> MRSDGRKEDQLRPVSIQRDFLEYPEGSCLISFGKTKVICTASVIENVPNWLKGKGQGWITAEYSMLPRATQQRTIRESVQGRIGGRTHEIQRMIGRAMRTA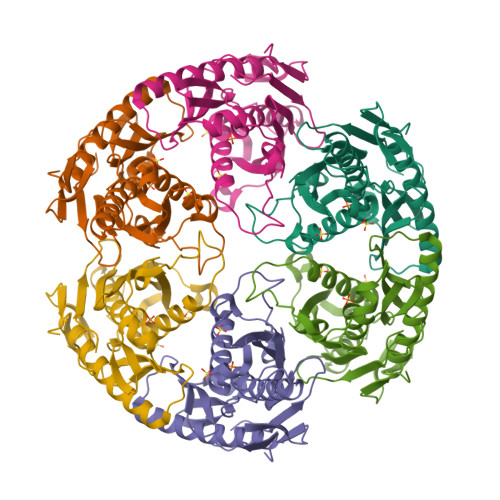VELTKIGERTIWVDCDVIQADGGARTAAITGAFVAVADAIIKLHKEGIIEETPIKDFVAAVSVGIVNDRILLDLNFEEDSAAQVDMNVVGTGSGRLSEVHTMGEEYSFTKDELIKMLDLAQKGINELIELQKKLYVIQDGKWERSELKEVSSTT> SNANKSAGTQAEKTATDLPPGFSGKAGSANATPGTKGLDGPTPLADGSFDATIFGPAKELKSADDILNVHRRNAKDPFAVGAVDAPLVITEFSDFECPFCARWSNQTEPTLMEEYVSKGLVRIEWNDLPVNGEHALAAAKAGRAAAAQGKFDEFRKALFEASRNVSGHPNNTLKDFERFARNAGVKDMERFSREAQDSTYDEVLTKAADYAHGLGVSGTPAFVVGTQYISGAQPTEEFIKVIESELKKSPTFSTPSSHQN

Using genetic suppressor, structural, and biochemical analyses, we provide evidence to support that C. diphtheriae encodes TsdA as a compensatory thiol-disulfide oxidoreductase safeguarding oxidative protein folding in this actinobacterium against thermal stress. The overall structure represents a typical DsbA/MdbA protein family fold, including a thioredoxin-like domain and an α-helical domain, which are found in actinobacterial MdbA proteins. Clearly, these results altogether demonstrate that TsdA is a potent thiol-disulfide oxidoreductase that when expressed at a sufficient level is capable of replacing the major oxidative protein-folding enzyme MdbA in C. diphtheriae, and that its enzymatic activity requires the conserved catalytic CxxC motif. Given our finding that tsdA expression is upregulated under heat stress, we propose that TsdA is a stress-adaptive thiol-disulfide oxidoreductase that protects corynebacteria under stress conditions.

To reveal the structural basis for the potential thiol-disulfide oxidoreductase activity of TsdA, we determined the C. diphtheriae wild-type TsdA structure by X-ray crystallography refracted to 1.45 Å atomic resolution with R-work and R-free factors equal to 11.4 and 15.3 %, respectively. The structure is a single continuous amino acid chain covering 38 to 282 residues of the protein (full length MW of 31 kDa). Despite using a recombinant protein lacking its transmembrane domain (1–32) for crystallization, four N-terminal and seven C-terminal residues are not visible in the structure, most likely due to flexibility of these fragments. The thioredoxin-like domain (residues 54 to 160 and 230 to 282) consists of a five-strand β-sheet in an order of β1↑- β3↓- β2↓- β4↑- β5↓ and six flanking helices (one 310-helix, ƞ1, and five α-helices, α2-4 and α9-10). The thioredoxin-like domain is separated by the amino acid segment 161 to 229 of the α-helical domain. The conserved catalytic CPFC motif, residues 126 to 129, forms the active site together with a conserved cis-Pro loop (residues T248 and P249). The C126 residue is located at the N-terminal end of the kinked α-helix 126 to 136; such a location of the CXXC motif is characteristic of DsbA proteins. The cysteine sulfurs in the CXXC motif are 3.40 Å apart with clear separation of corresponding electron densities; thus, the structure represents a reduced form of the protein. In addition, the α-helical domain of TsdA is comprised of four α-helices. Of note, no additional cysteine residue is found in TsdA.METHYLMALONIC 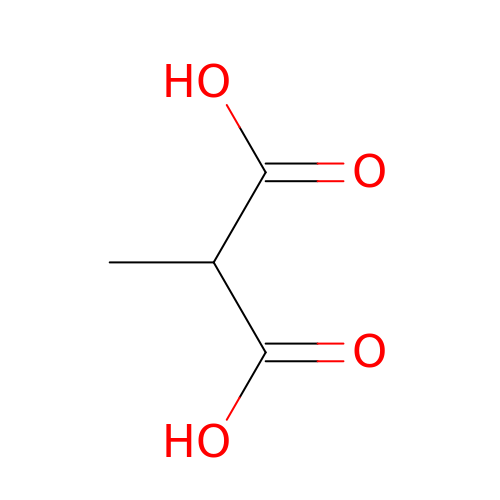ACID | C4 H6 O4 | ZIYVHBGGAOATLY-UHFFFAOYSA-N Here, we present structural and functional characterization of a putative polysaccharide deacetylase from Bacteroides ovatus (BoPDA) encoded in a CPS biosynthetic locus. Structural analysis of BoPDA revealed an atypical domain architecture that is unique to this enzyme, with a carbohydrate esterase 4 (CE4) superfamily catalytic domain inserted into a carbohydrate binding module (CBM). Additionally, BoPDA lacks the canonical CE4 His-His-Asp metal binding motif and our structures show it utilizes a noncanonical His-Asp dyad to bind metal ions. BoPDA is a lipoprotein unique to Bacteroides and likely has a role in the biosynthesis of capsular polysaccharides.

Four crystal structures of BoPDA bound to divalent cations were solved: to Co2+, Ni2+, Zn2+, and Cu2+ at 1.42 Å, 1.48 Å, 1.36 Å and 1.56 Å respectively. Co2+, Ni2+ and Zn2+ are the most common cations used by CE4 enzymes for catalysis. Our four metal-bound BoPDA crystal structures allowed us to investigate the metal-binding strategy of BoPDA given it lacks the canonical His-His-Asp triad. In the Co2+ bound BoPDA structure the divalent cation is coordinated with a His213-Asp102 dyad and four water molecules. The Co2+ ion is coordinated through typical octahedral geometry when validated using the CheckMyMetal (CMM) server, with acceptable values for all the CMM parameters. A composite omit map was generated for the BoPDA-Co2+ structure and it shows clear, defined density for the Co2+ cation and each water molecule modeled. Additionally, instead of four water molecules completing the metal binding site as in the BoPDA-Co2+ structure, there is a glycerol molecule (green, sticks) and 1 to 2 waters interacting with the Ni2+, Zn2+ or Cu2+ ion. Taken together, this suggests that the preferred metal for BoPDA is likely Co2+, and it may have reduced or no activity with Ni2+, Zn2+, or Cu2+. Through analysis of our structures, we hypothesize that Co2+ might be the catalytically relevant divalent ion for BoPDA enzymatic activity.

> GGCIRKLNLYQGDKDEDENKDNGKRRDVICETEFIYPFGNETADKEIEITIHLKADRQVGYLYTEIPTLKYNKDWLFLMTQDDCMHSAFSYTWAAIHGKPLSYIYYCDLAHLQNGDLPPDYYSLGKTLATTNGTGQEVRFSFGTTVAADDDLMNTQTWVQNGYTRDYFRFYKKTMLVWGNLQEMMNYGVSIAFHDLNLPDEDKTEDKLLAQFPVAQSMIREKLNNRTCKMLAEPNGDKNYIKAALRYDKIRTLCAQSGATKLYPFQENGDIEQVVIERAFYDPPEGSGLTNPDMIKAAILKEMENPKEERAAISIGAHNTDTGWVNFLEWLNDTYGRDGDDSMWFTNQEEYYEYYYYRLHSKPEIKQVNTHTWKLTLNLNGEDSAPFYYPSVTVNIFGLKMGDIESIKSNEDVTGLSYGDHKDFFMLNIDCRKYLAEHAENFVKRYEANPTDVSAKADANYFVNMLKDSDKKTELKKRIE(2S,4aR,6R,7S,8R,8aS)-7-(acetylamino)-6-({2-(acetylamino)-3-O-[2-(acetylamino)-2-deoxy-beta-D-glucopyranosyl]-4,6-O-[(1S)-1-carboxylic 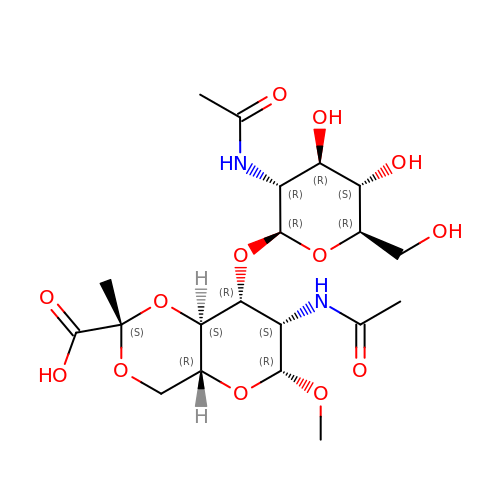acidethylidene]-2-deoxy-beta-D-mannopyranosyl}oxy)-8-{[2-(acetylamino)-2-deoxy-beta-D-glucopyranosyl]oxy}-2-methylhexahydro-2H-pyrano[3,2-d][1,3]dioxine-2-carboxylic acid | C20 H32 N2 O13 | HMXWDMHKOICGNH-MYXXRMNRSA-N>GSSHHHHHHSSGLVPGGSHMVSKGEENNMAVIKPDMKIKLRMEGAVNGHPFAIEGVGLGKPFEGKQSMDLKVKEGGPLPFAYDILTTVFCYGNMVFAKYPENIVDYFKQSFPEGYSWERSMNYEDGGICNATNDI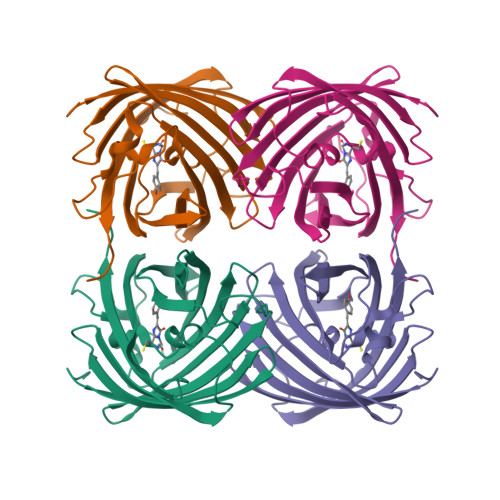TLDGDCYIYEIRFDGVNFPANGPVMQKRTVKWEPSTEKLYVRDGVLKGDVNTALSLEGGGHYRCDFKTTYKAKKVVQLPDYHFVDHHIEIKSHDKDYSNVNLHEHAEAHSGLPRQAMDELYK[6x]> MHLNPAEKEKLQIFLASELLLRRKARGLKLNYPEAVAIITSFIMEGARDGKTVAMLMEEGKHVLTRDDVMEGVPEMIDDIQAEATFPDGTKLVTVHNPIS;> NYIVPGEYRVAEGEIEINAGREKTTIRVSNTGDRPIQVGSHIHFVEVNKELLFDRAEGIGRRLNIPSGTAARFEPGEEMEVELTELGGNREVFGISDLTNGSVDNKELILQRAKELGYKGVE;> MKINRQQYAESYGPTVGDEVRLADTDLWIEVEKDYTTYGDEVNFGGGKVLREGMGENGTYTRTENVLDLLLTNALILDYTGIYKADIGVKDGYIVGIGKGGNPDIMDGVTPNMIVGTATEVIAAEGKIVTAGGIDTHVHFINPDQVDVALANGITTLFGGGTGPAEGSKATT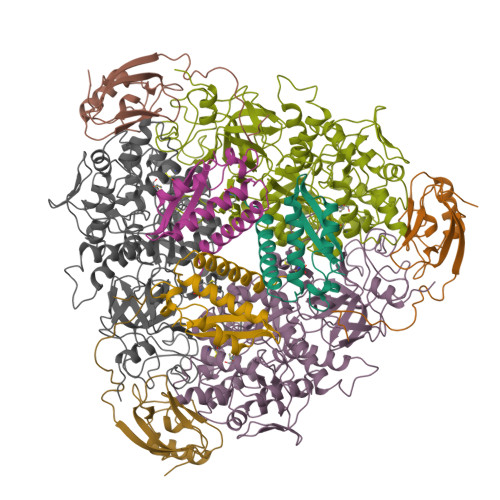VTPGPWNIEKMLKSTEGLPINVGILGKGHGSSIAPIMEQIDAGAAGLKIHEDWGATPASIDRSLTVADEADVQVAIHSDTLNEAGFLEDTLRAINGRVIHSFHVEGAGGGHAPDIMAMAGHPNVLPSSTNPTRPFTVNTIDEHLDMLMVCHHLKQNIPEDVAFADSRIRPETIAAEDILHDLGIISMMSTDALAMGRAGEMVLRTWQTADKMKKQRGPLAEEKNGSDNFRLKRYVSKYTINPAIAQGIAHEVGSIEEGKFADLVLWEPKFFGVKADRVIKGGIIAYAQIGDPSASIPTPQPVMGRRMYGTVGDLIHDTNITFMSKSSIQQGVPAKLGLKRRIGTVKNCRNIGKKDMKWNDVTTDIDINPETYEVKVDGEVLTCEPVKELPMAQRYFLF>[2x]MVKEYKTITQIAGPLIFVEKTEPVGYNEIVNI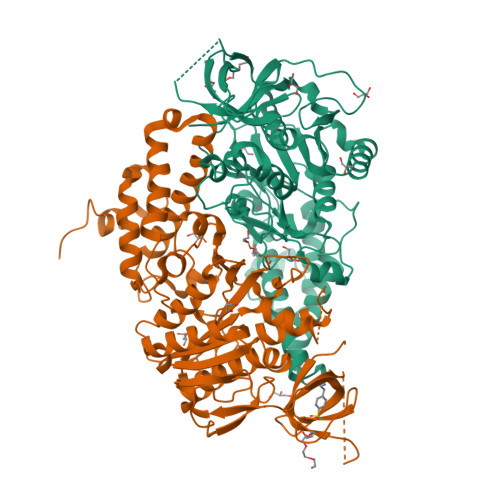KMGDGTVRRGQVLDSSADIVVVQVFEGTGGLDKDCGVIFTGETLKLPASVDLLGRILSGSGEPRDGGPRIVPDQLLDINGAAMNPYARLPPKDFIQTGISTIDGTNTLVRGQKLPIFSASGLPHAEIALQIARQASVPGSESAFAVVFAAMGITNEEAQYFMSDFEKTGALERAVVFLNLADDPAVERIVTPRMALTAAEYLAYEHGMHVLVILTDITNYAEALRQMGAARNEVPGRRGYPGYMYTDLATLYERAGIVKGAKGSVTQIPILSMPGDDITHPIPDLSGYITEGQIVVARELHRKGIYPPINVLPSLSRLMNSGIGAGKTREDHKAVSDQMYAGYAEGRDLRGLVAIVGKEALSERDTKFLEFADLFEDKFVRQGRNENRTIEDTLEIGWQILTHLPENQLGRIDNKYIQKYHPAHRKAK> GPLGSMSGIALSRLAQERKAWRKDHPFGFVAVPTKNPDGTMNLMNWECAIPGKKGTPWEGGLFKLRMLFKDDYPSSP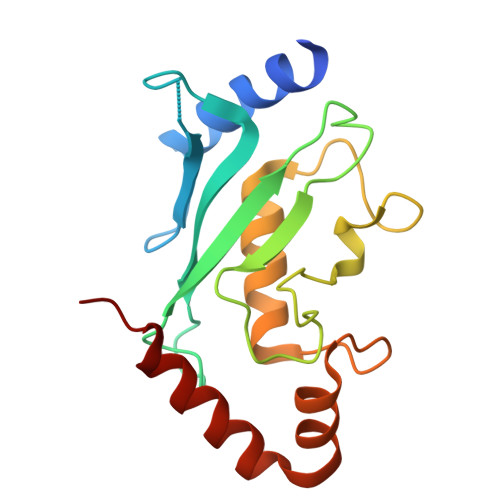PKCKFEPPLFHPNVYPSGTVCLSILEEDKDWRPAITIKQILLGIQELLNEPNIQDPAQAEAYTIYCQNRVEYEKRVRAQAKKFAPS> GAMGSMSAPSSVPPHKMANLHKLQRAWTLWYDSPSTYNTENWEMSLVPIMTVHSVEEFFVMLRYMKPLHALRTSSQYHFFQEGVKPMWEDPANKKGGKLWVNLDITSANGRSSNNNTSGTSAADGSAAEAKTDLDKAWENVLMATVGEYLDCVDKKDTPTEPFVTGIVMSKRKYHNRLAVWVSDASATDKIEALKKALTKEASLAPIASMVFTKHGEAS;> GS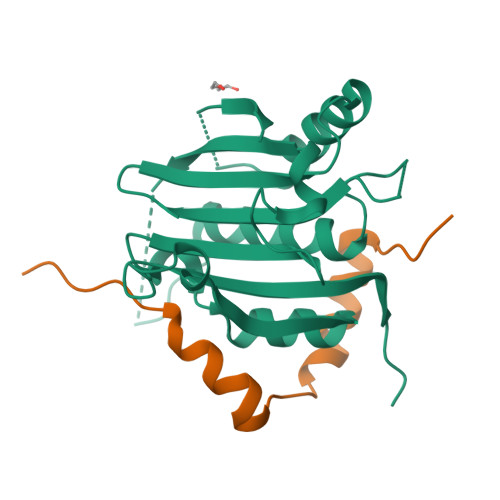PSVRTMYTREELLRIATLASAMDLGPEVLRKFDVIEVAEPVPTPKRRDAES> MNV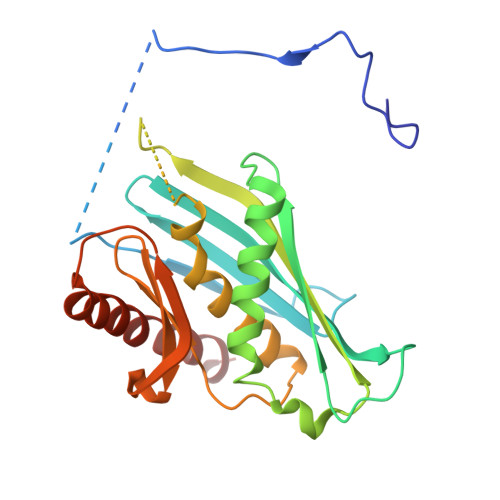QDRRRLLGPAAAKPMAFSNTTTHVPEKKSTDLTPKGNESEQELSLHTGFIENCNGSALVEARSLGHQTSLISAVYGPRSIRGSFTSQGTISIQLKNGLLEKYNTNELKEVSSFLMGIFNSVVNLSRYPKSGIDIFVYLTYDKDLTNNPQDDDSQSKMTSSQISSLIPHCITSITLALADAGIELVDMAGAGEANGTVVSFIKNGEEIVGFWKDDGDDEDLLECLDRCKEQYNRYRDLMISCLMNQET{5-methoxy-2-[(naphthalen-2-ylsulfonyl)carbamoyl]-1H-indol-1-yl}acetic acid | C22 H18 N2 O6 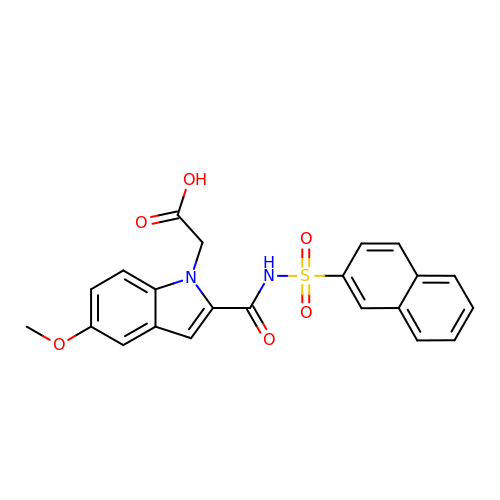S | VASHUENQUNBZFK-UHFFFAOYSA-N In Escherichia coli, the 14-cistron phn operon encoding carbon-phosphorus lyase allows for utilisation of phosphorus from a wide range of stable phosphonate compounds containing a C-P bond. The crystal structure of a core enzyme complex, Phn(GHIJ)2, revealed a symmetrical hetero-octamer consisting of a compact, central tetramer of the PhnI and PhnG subunits each interacting individually with the more distal PhnJ and PhnH subunits. Here, we show using single-particle cryogenic electron microscopy that PhnJ mediates binding of a double dimer of the ATP-binding cassette proteins, PhnK and PhnL, to the core complex. ATP hydrolysis induces drastic structural remodelling leading to opening of the core complex and reconfiguration of a metal-binding and putative active site located at the interface between the PhnI and PhnJ subunits.

An initial map generated using 901,800 particles resulted in a structure with an overall resolution of 2.2 Å (using the gold standard Fourier shell correlation (FSC) 0.143 cut-off criterion) of the C–P lyase core complex bound to a single PhnK subunit as previously observed. PhnK displayed a significantly lower resolution than the core PhnGHIJ complex, so we used 3D classification with signal subtraction to focus the refinement on PhnK and obtained a final class consisting of 50,323 particles at a resolution of 2.6 Å. This map had improved density for PhnK and allowed for tracing of the complete fold of the protein. Variability analysis revealed several distinct positions of PhnK representing a hinge-like motion of the ABC domain around the site of interaction. The specific interaction of PhnK with the CID of PhnJ is driven primarily by electrostatic interactions involving negatively charged residues on PhnJ (Glu149, Asp226, Asp228, and Asp229) and a positive patch on PhnK (Arg78, Arg82, and Arg116). These interactions are further stabilised by hydrophobic interaction between PhnJ Tyr158 and PhnK Tyr118. In a subset of 3D classes, additional EM density was visible near the P-loop of PhnK. The density overlaps partially with that of ATP inside NBD modules in ABC transporters, but the lack of high-resolution features suggests that any nucleotide binding is disordered and consequently that PhnK is not in a catalytically competent state. In summary, we conclude that when a single PhnK subunit binds to the C–P lyase core complex, it is structurally disordered and cannot engage in ATP hydrolysis. Moreover, and in contrast to previous observations, we observe no significant structural changes in the PhnGHIJ core complex, including the putative Fe4S4 cluster site, upon binding of a single subunit PhnK (rmsd = 0.5 Å).

>MHADTATRQHWMSVLAHSQPAELAARLNALNITADYEVIRAAETGLVQIQARMGGTGERFFAGDATLTRAAVRLTDGTLGYSWVQGRDKQHAERCALIDALMQQSRHFQNLSETLIAPLDADRMARIAARQAEVNASRVDFFTMVRGDNA[2x];>[2x]MTLETAFMLPVQDAQHSFRRLLKAMSEPGVIVALHQLKRGWQPLNIATTSVLLTLADNDTPVWLSTPLNNDIVNQSLRFHTNAPLVSQPEQATFAVTDEAISSEQLNALSTGTAVAPEAGATLILQVASLSGGRMLRLTGAGIAEERMIAPRLPECILHELTERPHPFPLGIDLILTCGERLLAIPRTTHVEVC;>MYVAVKGGEKAIDAAHALQESRRRGDTDLPELSVAQIEQQLNLAVDRVMTEGGIADRELAALALKQASGDNVEAIFLLRAYRTTLAKLAVSEPLDTTGMRLERRISAVYKDIPGGQLLGPTYDYTHRLLDFTLLANGEAPTLTTADSEQQPSPHVFSLLARQGLAKFEEDSGAQPDDITRTPPVYPCSRSSRLQQLMRGDEGYLLALAYSTQRGYGRNHPFAGEIRSGYIDVSIVPEELGFAVNVGELLMTECEMVNGFIDPPGEPPHFTRGYGLVFGMSERKAMAMALVDRALQAPEYGEHATGPAQDEEFVLAHADNVEVAGFVSHLKLPHYVDFQAELELLKRLQQEQNHG[2x];>MANLSGYNFAYLDEQTKRMIRRAILKAVAIPGYQVPFGGREMPMPYGWGTGGIQLTASVIGESDVLKVIDQGADDTTNAVSIRNFFKRVTGVNTTERTDDATVIQTRHRIPETPLTEDQIIIFQVPIPEPLRFIEPRETETRTMHALEEYGVMQVKLYEDIARFGHIATTYAYPVKVNGRYVMDPSPIPKFDNPKMDMMPALQLFGAGREKRIYAVPPFTRVESLDFDDHPFTVQQWDEPCAICGSTHSYLDEVVLDDAGNRMFVCSDTDYCRQQSEAKNQ[2x];> MNQPLLSVNNLTHLYAPGKGFSDVSFDLWPGEVLGIVGESGSGKTTLLKSISARLTPQQGEIHYENRSLYAMSEADRRRLLRTEWGVVHQHPLDGLRRQVSAGGNIGERLMATGARHYGDIRATAQKWLEEVEIPANRIDDLPTTFSGGMQQRLQIARNLVTHPKLVFMDEPTGGLDVSVQARLLDLLRGLVVELNLAVVIVTHDLGAARLLADRLLVMKQGQVVESGLTDRVLDDPHHPYTQLLVSSVLQNHHHHHH> MSAVALPRVSGGHDEHGHLEEFRTDPIGLMQRVRDECGDVGTFQLAGKQVVLLSGSHANEFFFRAGDDDLDQAKAYPFMTPIFGEGVVFDASPERRKEMLHNAALRGEQMKGHAATIEDQVRRMIADWGEAGEIDLLDFFAELTIYTSSACLIGKKFRDQLDGRFAKLYHELERGTDPLAYVDPYLPIESFRRRDEARNGLVALVADIMNGRIANPPTDKSDRDMLDVLIAVKAETGTPRFSADEITGMFISMMFAGHHTSSGTASWTLIELMRHRDAYAAVIDELDELYGDGRSVSFHALRQIPQLENVLKE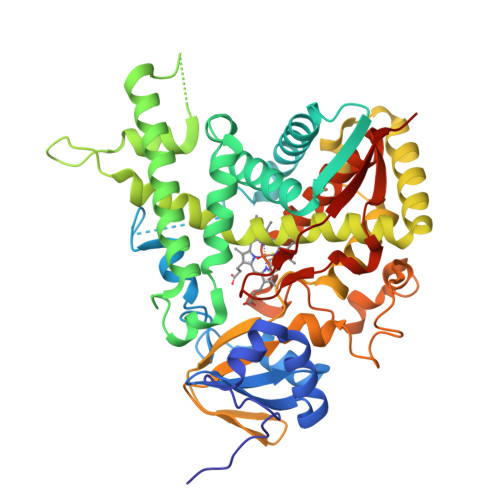TLRLHPPLIILMRVAKGEFEVQGHRIHEGDLVAASPAISNRIPEDFPDPHDFVPARYEQPRQEDLLNRWTWIPFGAGRHRCVGAAFAIMQIKAIFSVLLREYEFEMAQPPESYRNDHSKMVVQLAQPACVRYRRRTGVHHHH> SEDPVFTFGLIADVQYADIEDGENYLRTRRRYYRGSADLLRDAVLQWRRERVQCVVQLGDIIDGHNRRRDASDRALDTVMAELDACSVDVHHVWGNHEFYNFSRPSLLSSRLNSAQRTGTDTGSDLIGDDIYAYEFSPAPNFRFVLLDAYDLSVIGREEESEKHTHSWRILTQHNHNLQDLNLPPVSVGLEQRFVKFNGGFSEQQL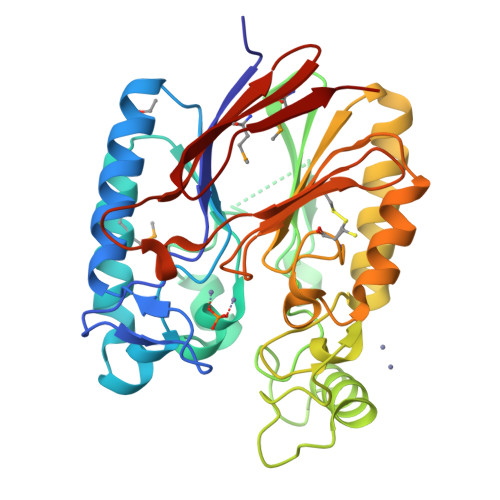QWLDAVLTLSDHKQERVLIFSHLPVHPCAADPICLAWNHEAVLSVLRSHQSVLCFIAGHDHDGGRCTDSSGAQHITLEGVIETPPHSHAFATAYLYEDRMVMKGRGRVEDLTITYS> YGKPGPDGPDGPKGKPGPKGKPG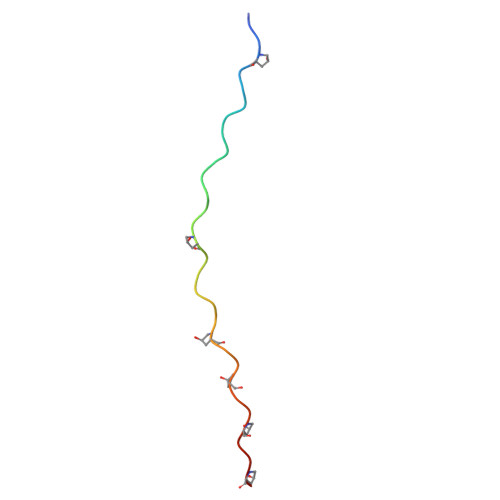KPGKPGKPG> MAQRGIREYDAKNLLARYLPEYLDDFSYKGNLALVGPETDIEGLEAENPWLKTTRLVVKPDQLFGKRGKLGLVLLDADWEEAKEYLNEKMGLEVTIGGITGRLSYFLIEPFTPHKEEYYVAISSDYEGDNIFFSMDGGVGVEENWEKVISIHVDSLEGIDALDVGSKLPAELGDKRALVEEFITALWRFYSDTGFAYVEINPFTFSGRGIVPLDMVAKLDDAEEYWQKKRWSELAFPEPFGRTPSKEELFIKEIDSKTGASLKLTILNPEGRVWTMVAGGGASVIYADTICDLGHADEMANYGEYSGDPNTEETYHYTCTILDLMTRSKNPNGKVLLIGGAIANFTDVAKTFKGVVMALEEYQQK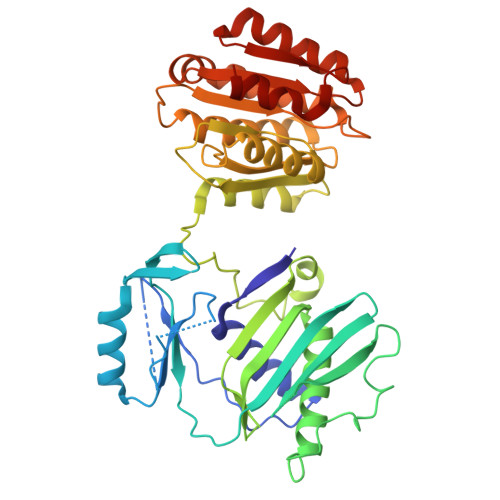LQEADIEIYVRRGGPNYEQGLKLMRDLGKRLGVPIQVHGPETHMTRIVPLALEENQ> MGSSHHHHHHSQDPNSMTTLTRQDLNFGQVVADVLCEFLEVAVHLILYVREVYPVGIFQKRKKYNVPVQMSCHPELNQYIQDTLHCVKPLLEKNDVEKVVVVILDKEHRPVEKFVFEITQPPLLSISSDS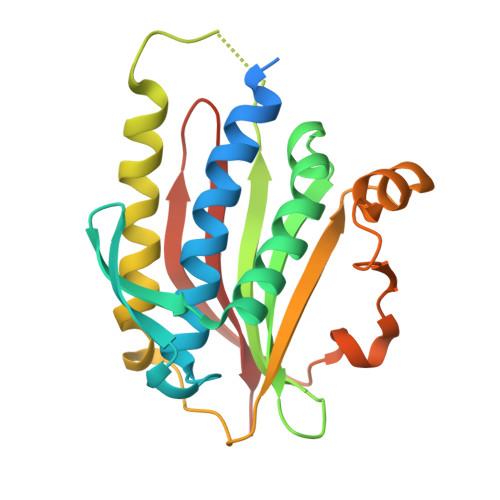LLSHVEQLLAAFILKISVCDAVLDHNPPGCTFTVLVHTREAATRNMEKIQVIKDFPWILADEQDVHMHDPRLIPLKTMTSDILKMQLYVEERAHKGS>[4x]MENLKKYLEVAKIAALAGGQVLKENFGKVKKENIEEKG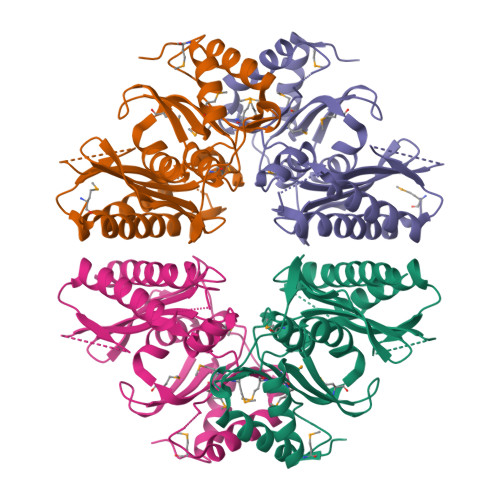EKDFVSYVDKTSEERIKEVILKFFPDHEVVGEEMGAEGSGSEYRWFIDPLDGTKNYINGFPIFAVSVGLVKGEEPIVGAVYLPYFDKLYWGAKGLGAYVNGKRIKVKDNESLKHAGVVYGFPSRSRRDISIYLNIFKDVFYEVGSMRRPGAAAVDLCMVAEGIFDGMMEFEMKPWDITAGLVILKEAGGVYTLVGEPFGVSDIIAGNKALHDFILQVAKKYMEVAV> MATLEITDIALVQPSHQPLSNDQTLSLSHLDNDNNLHVSFRYLRVYSSSSSTVAGESPSAVVSASLATALVHYYPLAGSLRRSASDNRFELLCSAGQSVPLVNATVNCTLESVGYLDGPDPGFVERLVPDPTREEGMVNPCILQVTMFQCGGWVLGASIHHAICDGLGASLFFNAMAELARGATKISIEPVWDRERLLGPREKPWVGAPVRDFLSLDKDFDPYGQAIGDVKRDCFFVTDDSLDQLKA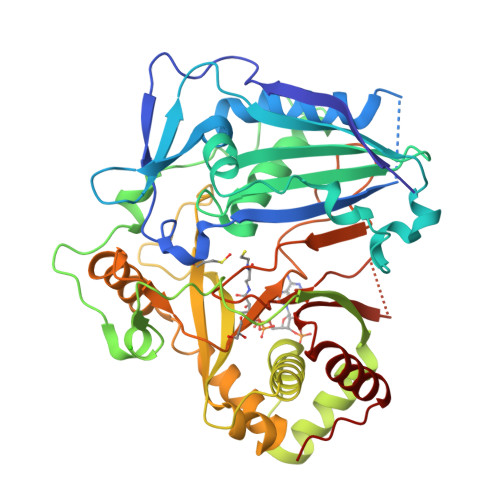QLLEKSGLNFTTFEALGAYIWRAKVRAAKTEEKENVKFVYSINIRRLMNPPLPKGYWGNGCVPMYAQIKAGELIEQPIWKTAELIKQSKSNTSDEYVRSFIDFQELHHKDGINAGTGVTGFTDWRYLGHSTIDFGWGGPVTVLPLSNKLLGSMEPCFFLPYSTDAAAGSKKDSGFKVLVNLRESAMPEFKEAMDKFHKGEFALS> MLSRASIRAYSSIPNSVKIAAKESATDLTKLSVIINNAGSKTGKSGVSHLLSKFTFLNNGAKSALRFTRESELLGGTFESKVTRDALILNTTFLKQDLPYYVEALGNVVSNTQFAPHEFNEIVLPTANAETKLANANPAFKGVEKLHEITFRRGLGNPLFYNESTPIKLEEVAQFSKEQFSGENISIVAEGANEEDLTKFVSESAFCYLPSSSSNGAKALPTNTFTGQEARVPSSGASSALIG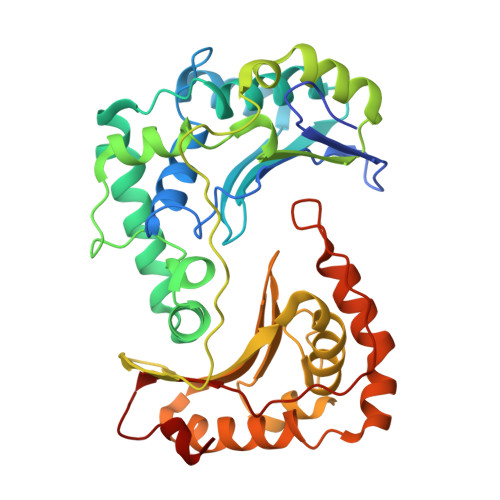IPVKPADFGKYEVLSAAIGTSTLPSTSTPLAQIPGATSHLYKYQDAGLFVISVSGEASQVAQGIKQAKSVAESVSSSALSEAVKAAELSVALQSTVDSPLNVKVVAEEAPISKFNYVAVGDLDVLPYADEL>[2x]MENLIGYVAAFLTTVSFLPQVLRVVMTKQTRDISRNMYIMFFLGVVLWFVYGILRSA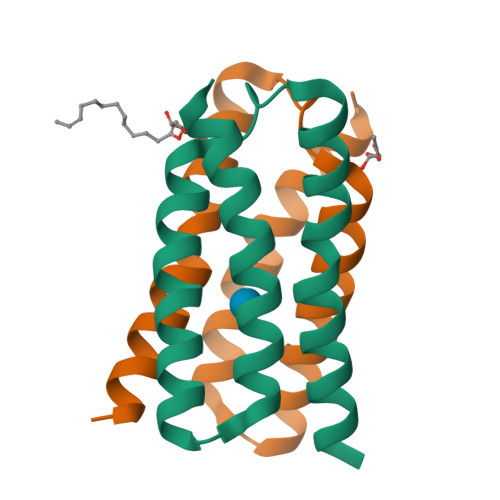LPIILANVVTLFFVTIILYYKLTEGNQTGSLEVLFQ>[2x]MRGSHHHHHHTDPQGDAAQKTDTSHHDQDHPTFNKITPNLAEFAFSLYRQLAHQSNSTNIFFSPVSIATAFAMLSLGTKADTHDEILEGLNFNLTEIPEAQIHEGFQELLRTLNQPDSQLQLTTGNGLFLSEGLKLVDKFLEDVKKLYHSEAFTVNFGDTEEAKKQINDYVE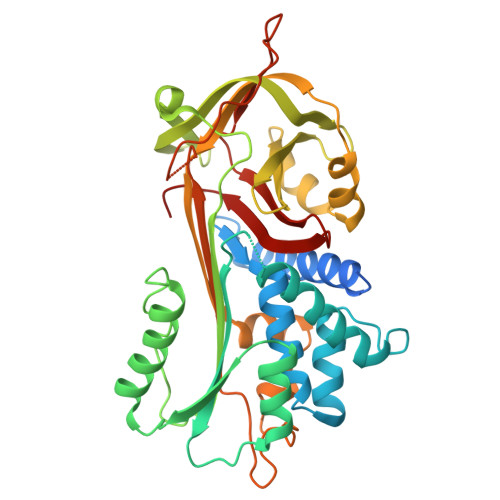KGTQGKIVDLVKELDRDTVFALVNYIFFKGKWERPFEVKDTEEEDFHVDQVTTVKVPMMKRLGMFNIQHCKKLSSWVLLMKYLGNATAIFFLPDEGKLQHLENELTHDIITKFLENEDRRSASLHLPKLSITGTYDLKSVLGQLGITKVFSNGADLSGVTEEAPLKLSKAVHKAVLTWDEKGTEAAGAMFLEAIPMSIPPEVKFNKPFVFLMIEQNTKSPLFMGKVVNPTQK> ADVTITVNGKVVA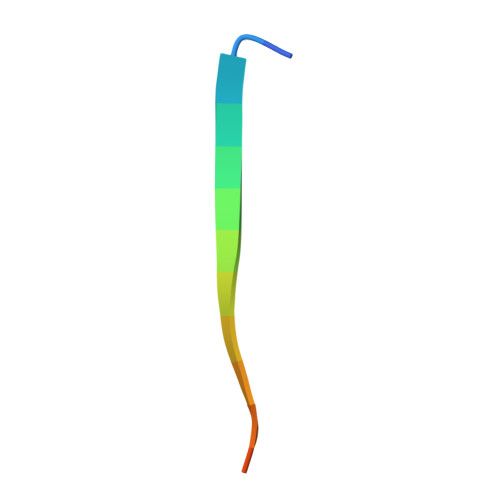KP>[4x]AYMFSDRSTSLSIEEERFLDAAEYGNIPVVRKMLEECHSLNVNCVDYMGQNALQLAVANEHLEITELLLKKENLSRVGDALLLAISKGYVRIVEAILSHPAFAEGKRLATSPSQSELQQDDFYAYDEDGTRFSHDVTPIILAAHCQEYEI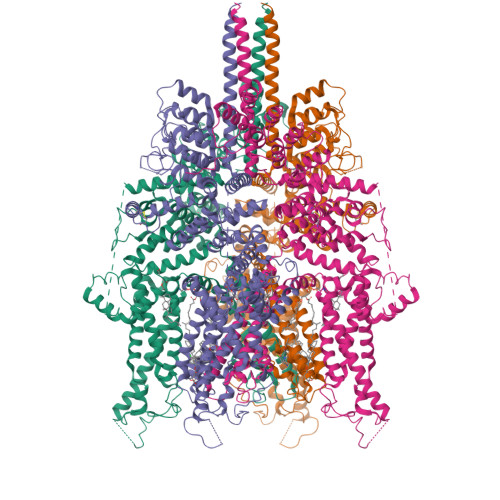VHTLLRKGARIERPHDYFCKCNDCNQKQKHDSFSHSRSRINAYKGLASPAYLSLSSEDPVMTALELSNELAVLANIEKEFKNDYKKLSMQCKDFVVGLLDLCRNTEEVEAILNGDVETLQSGDHGRPNLSRLKLAIKYEVKKFVAHPNCQQQLLSIWYENLSGLRQQTMAVKFLVVLAVAIGLPFLALIYWFAPCSKMGKIMRGPFMKFVAHAASFTIFLGLLVMNAADRFEGTKLLPNETSTDNAKQLFRMKTSCFSWMEMLIISWVIGMIWAECKEIWTQGPKEYLFELWNMLDFGMLAIFAASFIARFMAFWHASKAQSIIDANDTLKDLTKVTLGDNVKYYNLARIKWDPSDPQIISEGLYAIAVVLSFSRIAYILPANESFGPLQISLGRTVKDIFKFMVIFIMVFVAFMIGMFNLYSYYIGAKQNEAFTTVEESFKTLFWAIFGLSEVKSVVINYNHKFIENIGYVLYGVYNVTMVIVLLNMLIAMINSSFQEIEDDADVEWKFARAKLWFSYFEEGRTLPVPFNLVPSPKSLFYLLLKLKKWISELFQGHKKGFQEDAEMNKINEEKKLGILGSHEDLSKLSLDKKQVGHNKQPSIRSSEDFHLNSFNNPPRQYQKIMKRLIKRYTTQAQIDKESDEVNEGELKEIKQDISSLRYELLEEKSQNTEDLAELIRELGEKLSMEPNQEETNR>MSKQPMTPFEAIGGEQCIEILVDTFASYVSKHPDLSPIFPDDLTETARKQKQ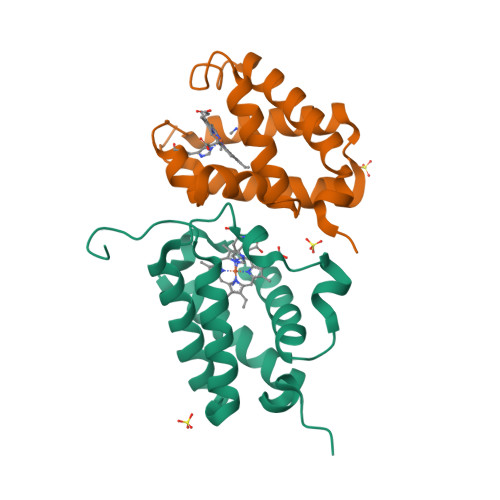FLTQYLGGPNLYTEEHGHPMLRARHLPFEITPKRAEAWLSCMEQAMDDTGVHGHIREFVFERLALTAQHMVNTPNETGEI[2x]RNF213, also known as ‘mysterin’, is the major susceptibility gene for Moyamoya disease (MMD), a cerebrovascular disorder characterized by arterial occlusions and abnormal blood vessel generation. Notably, with a mass of 591 kDa, RNF213 is the largest E3 ubiquitin ligase in the human proteome. It combines RING and AAA (ATPase associated with a variety of cellular activities) domains in a single polypeptide, making it a unique E3 machine in the ubiquitination system. As seen in the high-resolution cryo-EM structure, the 584 kDa RNF213 protein adopts an intricately intertwined fold that is organized into three major modules, namely an N-terminal stalk, a dynein-like core with six AAA units, and a multidomain E3 module.

Consistent with this, the full-length mouse RNF213 (584 kDa, 5148 residues) analyzed in the present study is a stable protein that could be efficiently produced in insect cells and analyzed by single-particle cryo-EM. The final atomic models of wildtype (wt) RNF213 and the R4753K MMD mutant comprise residues 476–5148, contain >80% of all side chains and were resolved at an average resolution of 3.2 Å and 3.1 Å, respectively, with the best-refined regions reaching 2.8 Å. Contrary to this, the present structure demonstrates that the protein encodes six AAA units within a single polypeptide chain. Analysis of individual ATPase motifs revealed that in RNF213 only AAA3 and AAA4 are catalytically competent, bearing all functional motifs. Moreover, the cryo-EM density unambiguously revealed a co-purified ATP molecule that is bound to AAA2. Consistent with the unexpected density, AAA2 contains a proper nucleotide binding site, but lacks catalytic residues (Walker B, sensor I) required for ATP hydrolysis. Instead, residues from both AAA2 and AAA3 tightly coordinate ATP, making the nucleotide a molecular glue tethering the two domains. At the edge of IR5, Tyr3078 reaches over toward the active site of AAA4, sterically blocking nucleotide binding. Together, the two insertions IR3 and IR5, which are amongst the most conserved RNF213 protein stretches, should hinder nucleotide binding to AAA3 and AAA4, diminishing RNF213 ATPase activity. We thus presume that the current cryo-EM structure reflects the auto-inhibited form of the RNF213 ATPase. The E3-RING, inserted between the two ultimate helices of the E3-back, contains a C4HC3 motif coordinating two Zn2+ ions in a cross-braced arrangement.

> XXXXXXXXXXXXXXXXXXXXXXXXXXXXXXXXXXXXXXXXXXXXXXXXXXXXXXXXXXXXXXXXXXXKLTLGLSILFMVEAAEFTVPKKDLDSLCYLLIPSAGSPEALHSDLSPVLRIRQRWRIYLTNLCLRCIDERCDRWLGILPLLHTCMQKSPPKKNSKSQPEDTWAGLEGISFSEFRDKAPTRSQPLQFMQSKMALLRVDEYLFRSWLSVVPLESLSSYLENSIDYLSDVPVRVLDCLQGISYRLPGLRKISNQNMKKDVENVFKMLMHLVDIYQHRIFGENLLQIYLTECLTLHETVCNITANHQFFEIPALSAELICKLLELSPPGHTDEGLPEKSYEDLVTSTLQEALATTRNWLRSLFKSRMLSISSAYVRLTYSEEMAVWRRLVEIGFPEKHGWKGSLLGDMEGRLKQEPPRLQISFFCSSQCRDGGLHDSVSRSFEKCVIEAVSSACQSQTSVLEGLSCQDLQKFGTLLSAVITKSWPVHNGEPVFDVDEIFKYLLKWPDVRQLFELCGTNEKIIDNITEEGRQLMATAESVFQKVAGELENGTIVVGQLELILEHQSQFLDIWNLNRRRLPSQEKACDVRSLLKRRRDDLLFLKQEKRYVESLLRQLGRVKHLVQVDFGNIEIIHSQDLSNKKLNEAVIKLPNSSSYKRETHYCLSPDIREMASKLDSLKDSHIFQDFWQETAESLNTLDKDPRELKVSLPEVLEYLYNPCYDNFYTLYENLKSGKITFAEVDAIFKDFVDKYDELKNDLKFMCTMNPQDQKGWISERVGQIKEYHTLHQAVSSAKVILQVRRALGVTGDFSVLNPLLNFADSFEDFGNEKLDQISPQFIKAKQLLQDISEPRQRCLEELARQTELVAWLHKALEDINELKVFVDLASISAGENDIDVDRVACFHDAVQGYASLLYKMDERTNFSDFMNHLQELWRALDNDQHLPDKLKDSARNLEWLKTVKESHGSVELSSLSLATAINSRGVYVIEAPKDGQKISPDTVLRLLLPDGHGYPEALRTYSTEELKELLNKLMLMSGKKDHNSNTEVEKFSEVFSNMQRLVHVFIKLHCAGNMLFRTWTAKVYCCPDGGIFMNFGLELLSQLTEKGDVIQLLGALCRQMEDFLDNWKTVVAQKRAEHFYLNFYTAEQLVYLSSELRKPRPSEAALMMLSFIKGKCTVQDLVQATSACESKADRYCLREVMKKLPQQLLSEPSLMGKLQVIMMQSLVYMSAFLPHCLDLDALGRCLAHLATMGGTPVERPLPKGLQAGQPNLILCGHSEVLPAALAIYMQAPRQPLPTFDEVLLCTPATTIEEVELLLRRCLTSGSQGHKVYSLLFADQLSYEVGCQAEEFFQSLCTRAHREDYQLVILCDAAREHCYIPSTFSQYKVPLVPQAPLPNIQAYLQSHYQVPKRLLSAATVFRDGLCVGIVTSERAGVGKSLYVNTLHTKLKAKLRDETVPLKIIRLTEPHLDENQVLSALLPFLKEKYQKMPVIFHIDISTSVQTGIPIFLFKLLILQYLMDINGKIWRRSPGHLYLVEIPQGLSVQPKRSSKLNARAPLFKFLDLFPKVTCRPPKEVIDMELTPERSHTDPAMDPVEFCSEAFQRPYQYLKRFHQQQNLDTFQYEKGSVEGSPEECLQHFLIYCGLINPSWSELRNFAWFLNCQLKDCEASIFCKSAFTGDTLRGFKNFVVTFMILMARDFATPTLHTSDQSPGRQSVTIGEVVEEDLAPFSLRKRWESEPHPYVFFNGDHMTMTFIGFHLETNNNGYVDAINPSNGKVIKKDVMTKELFDGLRLQRVPFNIDFDNLPRYEKLERLCLALGIEWPIDPDETYELTTDNMLKILAIEMRFRCGIPVIIMGETGCGKTRLIKFLSDLKRGSVEAETMKLVKVHGGTTPSMIYSKVKEAERTAFSNKAQHKLDTILFFDEANTTEAVSCIKEILCDRTVDGEHLHEDSGLHIIAACNPYRKHSQEMILRLESAGLGYRVSAEETADRLGSIPLRQLVYRVHALPPSLIPLVWDFGQLNDSAEKLYIQQIVQRLVDSVSVNPSETCVIADVLSASQMFMRKRENECGFVSLRDVERCVKVFRWFHDHSDMLLKELDKFLHESSDSTHTFERDPVLWSLVMAIGVCYHASLEEKASYRTAIARCFPKPYNSSRAILDEVTHVQDLFLRGAPIRTNIARNLALKENVFMMVICIELKIPLFLVGKPGSSKSLAKIIVADAMQGQAAFSELFRCLKQVHLVSFQCSPHSTPQGIISTFKQCARFQQGKDLGQYVSVVVLDEVGLAEDSPKMPLKTLHPLLEDGCIEDDPAPYKKVGFVGISNWALDPAKMNRGIFVSRGSPNEKELIESAEGICSSDRLVQDKIRGYFAPFAKAYETVCQKQDKEFFGLRDYYSLIKMVFAKAKASKRGLSPQDITHAVLRNFSGKDNIQALSIFTASLPEARYKEEVSTVELIKQNIYPGPQASSRGLDGAESRYLLVLTRNYVALQILQQTFFEGQQPEIIFGSSFPQDQEYTQICRNINRVKICMETGKMVVLLNLQNLYESLYDALNQYYVYLGGQKYVDLGLGTHRVKCRVHTAFRLIVIEEKDVVYKQFPVPLINRLEKHYLDMNTVLQPWQKSIVQELQQWAHEFADVKADQFIARHKYSPADVFIGYHSDACASVVLQAVERQGCRDLTEELYRKVSEEARSILLDCATPDAVVRLSGSSLGSFTAKQLSQEYYYAQQHNSFVDFLQAHLRMTHHECRAVFTEITTFSRLLTGNDCDVLASELRGLASKPVVLSLQQYDTEYSFLKDVRSWLTNPGKRKVLVIQADFDDGTRSAQLVASAKYTAINEINKTQGTKDFVFVYFVTKLSRMGSGTSYVGFHGGLWRSVHIDDLRRSTIMASDVTKLQNVTISQLFKPEDKPEQEEMEIETSQSKELAEEQMEVEDSEEMKKASDPRSCDCSQFLDTTRLVQSCVQGAVGMLRDQNESCARNMRRVTILLDLLNEDNTRNASFLRESKMRLHVLLNKQEENQVRSLKEWVTREAANQDALQEAGTFRHTLWKRVQDVVTPILASMIAHIDRDGNLELLAQPDSPAWVQDLWMFIYSDIKFLNISLVLNNTRSNSEMSFILVQSHMNLLKDAYNAVPFSWRIRDYLEELWVQAQYITDTEGLSKKFVEIFQKTPLGVFLAQFPVAQQQKLLQSYLKDFLLLTMKVSSREELMFLQMALWSCLRELQEASGTPDETYKFPLSLPWVHLAFQHFRTRLQNFSRILTIHPQVLSSLSQAAEKHSLAGCEMTLDAFAAMACAEMLKGDLLKPSPKAWLQLVKNLSTPLELVCSEGYLCDSGSMTRSVIQEVRALWNRIFSIALFVEHVLLGTESHIPELSPLVTTYVSLLDKCLEEDSNLKTCRPFVAVMTTLCDCKDKASKKFSRFGIQPCFICHGDAQDPVCLPCDHVYCLRCIQTWLIPGQMMCPYCLTDLPDKFSPTVSQDHRKAIEKHAQFRHMCNSFFVDLVSTMCFKDNTPPEKSVIDTLLSLLFVQKELLRDASQKHREHTKSLSPFDDVVDQTPVIRSVLLKLLLKYSFHEVKDYIQNYLTQLEKKAFLTEDKTELYLLFISCLEDSVHQKTSAGCRNLEQVLREEGHFLRTYSPGLQGQEPVRIASVEYLQEVARVRLCLDLAADFLSELQEGSELAEDKRRFLKHVEEFCTRVNNDWHRVYLVRKLSSQRGMEFVQSFSKQGHPCQWVFPRKVIAQQKDHVSLMDRYLVHGNEYKAVRDATAKAVLECKTLDIGNALMACRSPKPQQTAYLLLALYTEVAALYRSPNGSLHPEAKQLEAVNKFIKESKILSDPNIRCFARSLVDNTLPLLKIRSANSILKGTVTEMAVHVATILLCGHNQILKPLRNLAFYPVNMANAFLPTMPEDLLVHARTWRGLENVTWYTCPRGHPCSVGECGRPMQESTCLDCGLPVGGLNHTPHEGFSAIRNNEDRTQTGHVLGSPQSSGVAEVSDRGQSPVVFILTRLLTHLAMLVGATHNPQALTVIIKPWVQDPQGFLQQHIQRDLEQLTKMLGRSADETIHVVHLILSSLLRVQSHGVLNFNAELSTKGCRNNWEKHFETLLLRELKHLDKNLPAINALISQDERISSNPVTKIIYGDPATFLPHLPQKSIIHCSKIWSCRRKITVEYLQHIVEQKNGKETVPVLWHFLQKEAELRLVKFLPEILALQRDLVKQFQNVSRVEYSSIRGFIHSHSSDGLRKLLHDRITIFLSTWNALRRSLETNGEIKLPKDYCCSDLDLDAEFEVILPRRQGLGLCGTALVSYLISLHNNMVYTVQKFSNEDNSYSVDISEVADLHVISYEVERDLNPLILSNCQYQVQQGGETSQEFDLEKIQRQISSRFLQGKPRLTLKGIPTLVYRRDWNYEHLFMDIKNKMAQSSLPNLAISTISGQLQSYSDACEALSIIEITLGFLSTAGGDPGMDLNVYIEEVLRMCDQTAQVLKAFSRCQLRHIIALWQFLSAHKSEQRLRLNKELFREIDVQYKEELSTQHQRLLGTFLNEAGLDAFLLELHEMIVLKLKGPRAANSFNPNWSLKDTLVSYMETKDSDILSEVESQFPEEILMSSCISVWKIAATRKWDRQSRGGGHHHHHHHHHH> GMADTVLFEFLHTEMVAELW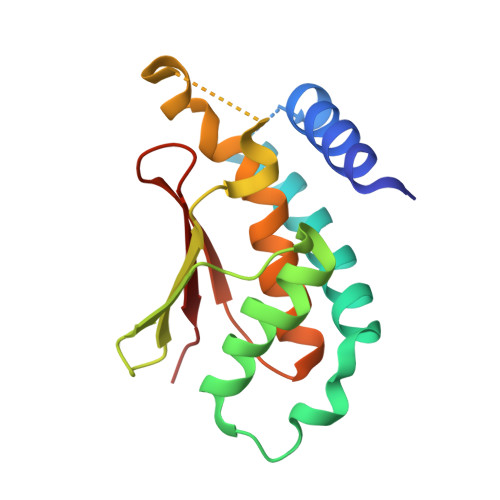AHDPDPGPGGQKMSLSVLEGMGFRVGQALGERLPRETLAFREELDVLKFLCKDLWVAVFQKQMDSLRTNHQGTYVLQDNSFPLLLPMASGLQYLEEAPKFLAFTCGLLRGALYTLGIESVVTASVAALPVCKFQVVIPKS> GPTKAPTKDGTSYKDLFLELYGKIKDPKNGYFSPDEGIPYHSIETLIVEAPDYGHVTTSEAFSYYVWLEAMYGNLTGNWSGVETAWKVMEDWIIPDSTEQPGMSSYNPNSPATYADEYEDPSYYPSELKFDTVRVGSDPVHNDLVSAYGPNMYLMHWLMDVDNWYGFGTGTQATFINTFQRGEQESTWETIPHPSIEEFKYGGPNGFLDLFTKDRSYARQWRYTNAPDAEGRAIQAVYWANKWAKEQGKGSAVASVVSKAAKMGDFLRNDMFDKYFMKIGAQDKTPATGYDSAHYLMAWYTSWGGGIGASWAWKIGCSHAHFGYQNPFQGWVSATQSDFAPKSSNGKRDWTTSYKRQLEFYQWLQSAEGAIAGGATNSWNGRYEKYPAGTSTFYGMAYVPHPVYADPGSNQWFGFQAWSMQRVMEYYLETGDSSVKNLIKKWVDWVMSEIKLYDDGTFAIPSDLEWSGQPDTWTGTYTGNPNLHVRVTSYGTDLGVAGSLANALATYAAATERWEGKLDTKARDMAAELVNRAWYNFYCSEGKGVVTEEARADYKRFFEQEVYVPAGWSGTMPNGDKIQPGIKFIDIRTKYRQDPYYDIVYQAYLRGEAPVLNYHRFWHEVDLAVAMGVLATYFPDGGGGGRPHHHHHHHHHHHH

As the major exoglucanase of cellulosome in C. thermocellum, Cel48S plays key roles and influences the activity and features of cellulosome to a great extent. Family 48 glucosyl hydrolases (GH48s) are exoglucanases that attack cellulose chains from the reducing ends to progressively release cellobiose molecule, thereby playing crucial roles in the hydrolysis of crystalline cellulose. Subsequently, Cel48S was defined as a family 48 cellulase because it contains a GH48-catalyzing domain with reducing end-acting cellobiohydrolase activity and a type I dockerin domain for assembly. The ctCel48S_CD protein adopted a typical (α/α)6 consisting of an inner core of six mutually parallel α-helixes connected by long loops, additional helices, or sheets to the six peripheral α-helixes.

A high-purity catalytic domain of the native Cel48S protein, termed ctCel48S_CD, was obtained from the extracellular proteins of C. thermocellum after one-step affinity purification. The crystal structure of the purified ctCel48S_CD protein was determined at 1.43Å obtaining final Rwork and Rfree values of 0.1601 and 0.1930, respectively. The crystal structure showed one molecule in an asymmetric unit. The structure of the ctCel48S_CD proteins was obtained without substrate binding. However, a long PEG molecule was observed in the substrate channel, which may mimic the structure of a cellulose chain. The ctCel48S_CD structure was well matched with the published rCel48S_CD structure, with a Cα RMSD of approximately 0.32 Å, especially for the residues responsible for substrate binding (i.e., T140, Q247, K301, Y302, W326, Y327, Y351, D520, W645, and H646). We observed conformational changes of three important residues: the substrate-binding residues R249 and Y431, and the catalytic residue E87. The side chain of E87 deviated approximately 3.7 Å from that of the substrate-bound rCel48S_CD, which resulted in an increasing distance (from 2.8 Å to 6.0 Å) between the carboxylate oxygen of E87 and C4 hydroxyl of glucosyl residues at subsite + 1. The side chain of residue R249 in the ctCel48S_CD structure showed apparent conflicts with the substrate based on the published rCel48S_CD-oligosaccharide complex structure. Because the ctCel48S_CD structure was substrate- and product-free compared with the published rCel48S_CD structure, these results indicated that the residue conformation of the Cel48S protein may differ as the substrate-binding status changes, indicating that induced-fit effects may occur between the enzyme and substrates.> MPREVEPSLSERQFVLQALQEGLRLDGRQLDQYRPLSLTFGDQYGVADVTFGKTRVLAKASAEVTVPYADRPLDGIFTIATELSPMTSPTFEVNRPTETEVLLSRLLEKTIRRSGALDTESLCLVAGQKCWSIRVDVHVMSHDGNLVDAACIAVVAALRHFRKPDTSIESGVLTIYTPAEREPVPLSWLHTPFCVTWSFFGDEGEIAVLDATWLEEQVRVGSCTISMNKHGEICQIAKLGGTPVEAVSLLQCTSIALTKVKEFSDLVDKKLAEDFKRRNPGGLLKELKAENDR;> MPLDTSTYKLALLRVDGRRWNELRRVHAQIRTQAAADGSSYLEMGHTKVMCVVTGPSEPGPRRGTGAGTTGGGGAGGAGGGGSGGQGKEAEVVVSIVIAGFSSVDRKRHGRNDKRIIEMQSTVANALSASLHTHLFPHSQITISLHVLSQDGSLLAALINAATLACVDAGIPMTDYVVACTAGSTSTYAANDENADPLLDLNHQEEQELPWLTVATLGESDKVAVLVCESRVQVSRLEGMLAVGVDGCKQIRAILDHVVRQKGRRMIREGAVEKGVSLDDMDED;> MATDAASAPHSLTFPRGIFAKLSPHPYLLRTLCPDPSNSSSTPQRTNGRRPNEARPFRVNLGSLSHAHGSALVRAGDTTVLCGVRGEVLPVERIPLFRQPDVNGSGIGATVGRGELKEYDLLVPNIELATGSAPQFLPGVPPTALAQTLSTRVYSLLHSTRLVSAEELRIWYRPVATNRSKEGEDVEMEEECQEESGEEQDRVVAYWVLYIDLVFLSFDGNPFDVAWAAVVAALRDTKLPVARWDPDREMVVCSKTETMKLTIKGLPIACSAAVFLEKEHGEVAVGEKNRHWILLDPDRLEESLCKEVITMVVDFSDGETRIRAIEKQGGTVFGREL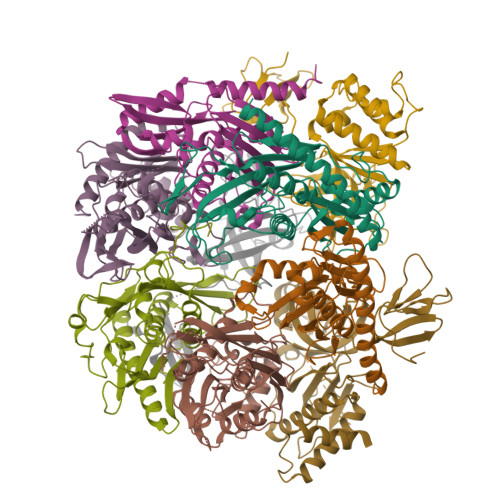IRSFALVAEDRWKVVKEVMK;> MTTTTATTAPEAALGVLPRADGSARYSHAGYTVTASVNGPIEAQRRDEHPYEAHVDVIVRPAAGVGGTRERHLESILQSSFAQIILVKSFPRSLIQIVLQVEESPENEYVNTKLVQASLNFAVMPALFQTAMLALLSAGVPMRATATATAIALASENGATKTLIDPSPRQVELAQSVHVFAFTSQDELLLAESEGDFTIKEWDAAYETAKNICCRPSPTMDGVQMMAIDDDRLVGPDLRHFIRSTMEAKVATDLHWKS;> MSAASSQHVLLSPAELAYLHASLSLTPPIRPDGRSPTQFRPLIAETGILPGANGSARVCFADGTEAIVGVKAEVEKTVSRSKEDEEVGLLVASAGDMDVDDEEGYAKVGADNRTGEASWVEITVEIPGVRDDDSGMVFLAQLLGEALLADGEFVKKLWINRRYHWKLYIDILLISPPLSYPLPLLSLTTHLALLSTRLPRLKSEGDEDPYFDDDWAVAPYLFPRSSSASKSSKSSPTQPTTRPPITLLVMAVGNNILFDPSKEELAVADVALAVSVTATDVDPDESDAQKETATATAGPDSADAAKRGRKLRLLSIRTIDPPSRLTPPGVPNSTNPAAIYGTTSSSGTNGNGQPQQKVESGKISEPIEPIEGVWRAPRGGAKRLVLGALVQKVLEKGGVVDEVLDALEGVELT;> MTDRRRINGPAGATIPPVYEDSGISEVKALKIRSRPSNIIRKIYLKTGVTPSASGSAYLELETSANSGVSGLKLSCTVHGPRSLPRSSPFSPHMVVSTHVKYAPFATKQRRGYLRDPTERDLGIHLEAALRGAIIADRWPKSGVDIIISIIEGDQDREASKTQGDEVWDMMNTLSGCITVASAALADAGIDCVDTVAGGVAALVQDSDGSPEIVVDPIPSEHRKILAACCVAYLPMRDEVTNLWFRGDLPASDMDLYTELVEKGIQASRSANRVLVDCLTETVG;> MSTTTRPFVLPGETIDPSLVPTHPKHPLRLGPGLRHVPPSDIIPTVAGQLITNLNKNSMWVEYNSQRYVPTQNDLVLAQVLRSTQDSYLCLITPHTPPATLPHLAFESATKKTRPQLQPGQLVYARVSLANRHMDPELECVNPSTGKADGLGPITGPGCVFEVSLGFARRLLMAKSREEGKVGVLEMLAGEDPSIGEAGAGLAFETAVGRNGRVWVGSEDVKTVIIVGRALQETDRGNLTIEGQRKLVRRLLREMR;> MPITIHAPLPPPRLHDEDSDVDMSSDSDSSSEGGVPLTSNLPSRAKPKSSLFTTTKSSSDIVTPGELITTSPQFMRGHGTYIPPGTTSIISSVAGTILRTNKLLSVRPLRARYTPEVGDLVVGRIIEVQARRWRVDVGSTQFASLPLSAINLPGGILRKRTETDELQMRSFFSEGDLLVAEVQGVYGDGGAVLHTRSLKYGKLRNGVFVAVSGMGGGGGVVRSRRQVWTLEGANGAGLIDVVLGVNGYVWIAKHTEDGPGEDPNASTKQVGITNLEEGMSANMYSSQNDRIEAETMREIARLRGVVMALVENGLRVDEDMVMRGYREAVEMALVSPEGPEDVYLGGERGRQLAAALTA;> MTTTQPTLALPGQLLGPISKYQPGPGTHVHESNLYSSLLGTVHVTQPARAPGPVKRLNRITPAPTPAELPTISVSAARPAGSAASGLVTGRKREILPEVGNIVLCRVIRITPRQAVVTILVCGDTVLDAEWQGLIRVQDIRATEKDRVKVYESFRPGDIVRAEVISLGDQANYYLSTARNELGVILATSEAGNTMYPVSWREYRDPITGLTELRKVAKPY>[2x]VQAVAVLKGDAGVSGVVKFEQASESEPTTVSYEIAGNSPNAERGFHIFEFGDATNGCVSAGPHFNPFKKTHGAPTDEVRHVGDMGNVKTDENGVAKGSFKDSLIKLIGPTSVVGRSVVIHAGQDDLGKGDTEESLKTGNAGPRPACGVIGLTN;>MTTNDTYEATYAIPMHCENCVNDIKACLKNVPGINSLNFD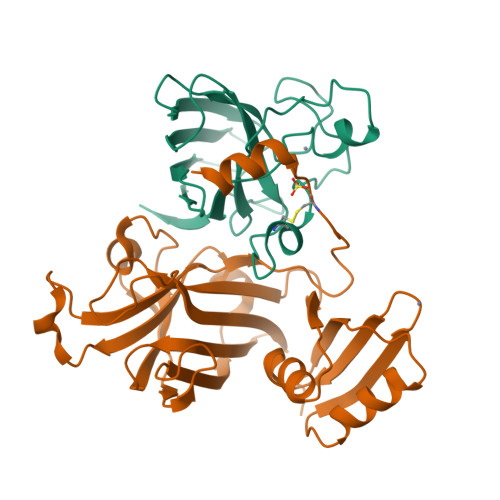IEQQIMSVESSVAPSTIINTLRNCGKDAIIRGAGKPNSSAVAILETFQKYTIDQKKDTAVRGLARIVQVGENKTLFDITVNGVPEAGNYHASIHEKGDVSKGVESTGKVWHKFDEPIECFNESDLGKNLYSGKTFLSAPLPTWQLIGRSFVISKSLNHPENEPSSVKDYSFLGVIARSAGVWENNKQVCACTGKTVWEERKDALANNIK[2x]> IIKVIK

High expression of PSMαs, which are four peptides of about 20-residues in length, increases virulence potential of methicillin-resistant S. aureus (MRSA). Amyloid aggregation plays roles in PSM activities in S. aureus. In the present study, we investigated the structure-function relationships of PSMαs and their short truncations.

To obtain atomic-level insights into the architecture of PSMα1 and PSMα4 fibrils, we computationally identified their amyloidogenic spine segments, and determined their high-resolution structures by means of X-ray microcrystallography. Segments PSMα1-IIKVIK and PSMα4-IIKIIK, both of which are conserved within naturally occurring PSM truncations, adopt the canonical cross-β fibril architecture, wherein pairs of β-sheets tightly mate through a dry interface, forming a steric zipper. Both structures belong to the class 1 of steric zippers, indicating that parallel β-sheets mate face-to-face in the fibrils formed by the PSMα1-IIKVIK and PSMα4-IIKIIK segments. Proline substitutions in these spine regions abolished fibril formation of the full-length PSMα1 and PSMα4. Structural indicators of fibril stability of the IIKVIK and IIKIIK segments, i.e., buried surface area and shape complementarity between sheets, calculated from the crystal structures, resemble those of eukaryotic steric-zipper structures. Specifically, the steric-zipper segment PSMα1-IIKVIK showed a peak at 1621 cm−1 corresponding to rigid cross-β amyloid fibrils, in accordance with the crystal structure. For example, fibrillation of PSMα1 promotes biofilm stability by preventing disassembly by matrix-degrading enzymes and mechanical stress. While PSMα3 forms cross-α fibrils and enhances toxicity against human cells, PSMα1 and PSMα4 form cross-β fibrils which likely play a role in stabilizing the biofilm matrix. The highly stable steric zipper structures, forming the spines of the cross-β fibrils, putatively serve as the building block cementing the biofilm and creating the rigidity that can explain the resistance of amyloid-containing biofilms. The atomic structures of the PSMα1 and PSMα4 derivatives offer templates for the design of anti-biofilm compounds.> MAHHHHHHVDDDDKMCSSNNLSKSNTSNSSKTSSSSKKMCSSNNLSKSNTSNSSKTSSSSKKITLTFWNLFTGEPAKTKVKEIIDQWNKENPNVQIVESVTENDAYKTKIKAAIAANEAPDIFQTWAGGFSQPFVEAGKVLQLDSYLNDGTKDQLLPGSFDNVTYNGKIYGIPFDQQASVLYINKELFDKYN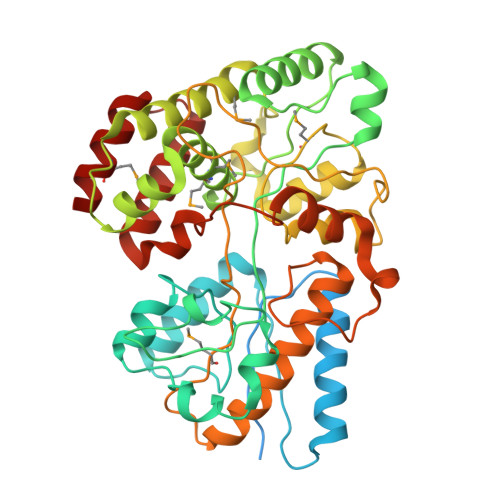VKVPTTFSELIDAIKTFKSKGVTPFALGEKDEWPGMWYYDMIALREGGVQLTRDALNGKASFDNQAFTDAAQKLQDMVNAGAFDSGFMGLTRDEATAEFNQGKAAMYFGGNFDAAAFVSDPSSLVKGKIEAVRFPTIEGGKGDPTEYIGGTVGALMVSANSKYKDEAVRAAKYLAKQLSDMDYLIATGLPAWKYDNIDQSKVDPLEIQIMNNIVANAKGSVPAWDIYLSGDAAQTHKDLVAQLFAKQITPEEYSKQMQQKINGK> VHHPPSYVAHLASDFGVRVFQQVAQASKDRNVVFSPYGVASVLAMLQLTTGGETQQQIQAAMGFKIDDKGMAPALRHLYKELMGPWNKDEISTTDAIFVQRDLKLVQGFMPHFFRLFRSTVKQVDFSEVERARF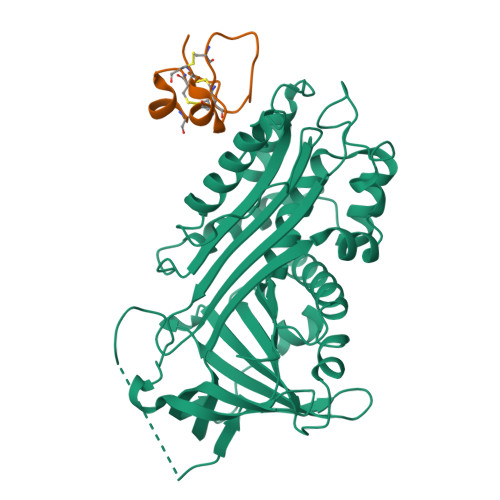IINDWVKTHTKGMISHLLGTGAVDQLTRLVLVNALYFNGQWKTPFPDSSTHRRLFHKSDGSTVSVPMMAQTNKFNYTEFTTPDGHYYDILELPYHGDTLSMFIAAPYEKEVPLSALTNILSAQLISHWKGNMTRLPRLLVLPKFSLETEVDLRKPLENLGMTDMFRQFQADFTSLSDQEPLHVALALQKVKIEVNESGTVASSSTAVIVSARMAPEEIIIDRPFLFVVRHNPTGTVLFMGQVMEP;> DQESCKGRCTEGFNVDKKCQCDELCSYYQSCCTDYTAECKPQVTRGDVFTM> SRKTYTLTDYLKNTYRLKLYSLRWISDHEYLYKQENNILVFNAEYGNSSVFLENSTFDEFGHSINDYSISPDGQFILLEYNYVKQWRHSYTASYDIYDLNKRQLITEERIPNNTQWVTWSPVGHKLAYVWNNDIYVKIEPNLPSYRITWTGKEDIIYNGITDWVYEEEVFSAYSALWWSPNGTFLAYAQFNDTEVPLIEYSFYSDESLQYPKTVRVPYPKAGAVNPTVKFFVVNTDSLSSVTNATSIQITAPASMLIGDHYLCDVTWATQERISLQWLRRIQNYSVMDICDYDESSGRWNCLVARQHIEMSTTGWVGRFRPSEPHFTL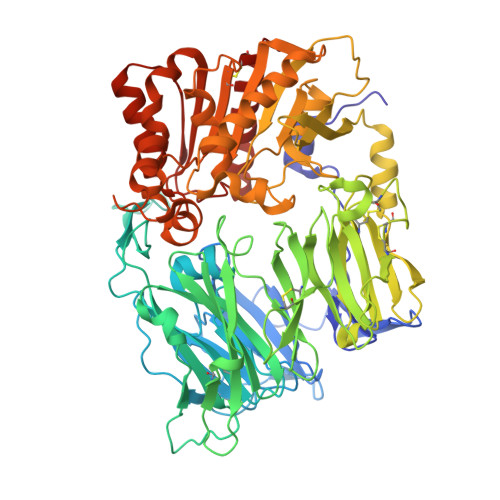DGNSFYKIISNEEGYRHICYFQIDKKDCTFITKGTWEVIGIEALTSDYLYYISNEYKGMPGGRNLYKIQLSDYTKVTCLSCELNPERCQYYSVSFSKEAKYYQLRCSGPGLPLYTLHSSVNDKGLRVLEDNSALDKMLQNVQMPSKKLDFIILNETKFWYQMILPPHFDKSKKYPLLLDVYAGPCSQKADTVFRLNWATYLASTENIIVASFDGRGSGYQGDKIMHAINRRLGTFEVEDQIEAARQFSKMGFVDNKRIAIWGWSYGGYVTSMVLGSGSGVFKCGIAVAPVSRWEYYDSVYTERYMGLPTPEDNLDHYRNSTVMSRAENFKQVEYLLIHGTADDNVHFQQSAQISKALVDVGVDFQAMWYTDEDHGIASSTAHQHIYTHMSHFIKQCFSLP>[6x]MSKSVFVGELTWKEYEARVAAGDCVLMLPVGALEQHGHHMCMNVDVLLPTAVCKRVAERIGALVMPGLQ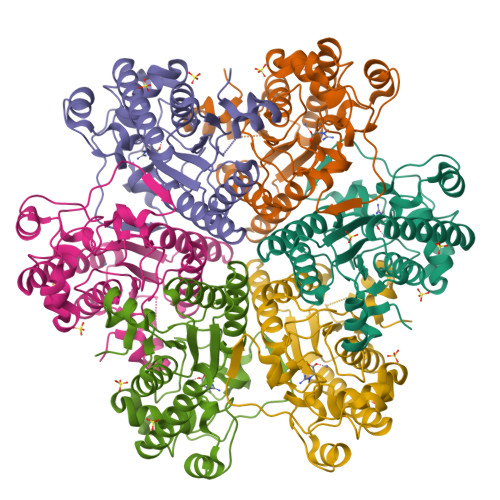YGYKSQQKSGGGNHFPGTTSLDGATLTGTVQDIIRELARHGARRLVLMNGHYQNSMFIVEGIDLALRELRYAGIQDFKVVVLSYWDFVKDPAVIQQLYPEGFLGWDIEHGGVFETSLMLALYPDLVDLDRVVDHPPATFPPYDVFPVDPARTPAPGTLSSAKTASREKGELILEVCVQGIADAIREEFPPT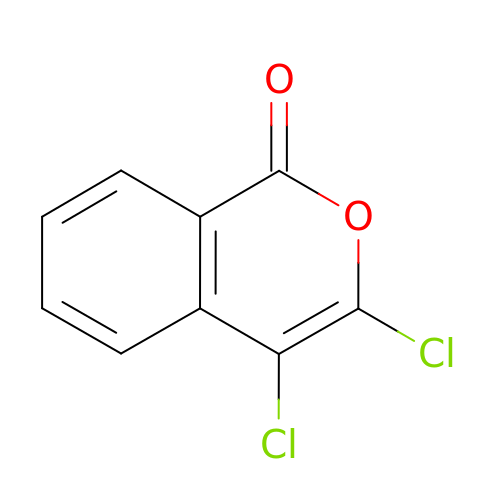3,4-DICHLOROISOCOUMARIN | C9 H4 Cl2 O2 | SUGXUUGGLDCZKB-UHFFFAOYSA-N>GSGSPLAQQIKNIHSFIHQAKAAGRMDEVRT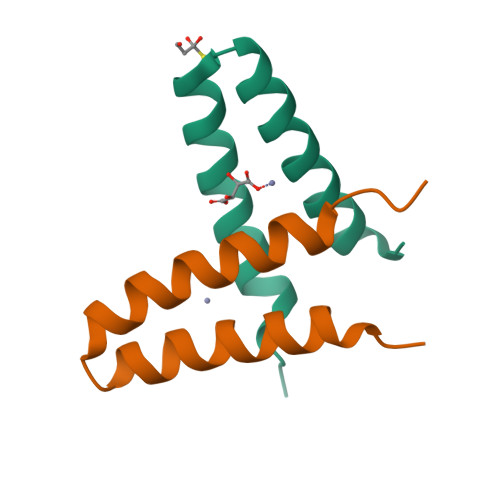LQENLHQLMHEYFQQSD[2x]>[2x]MAKKVTV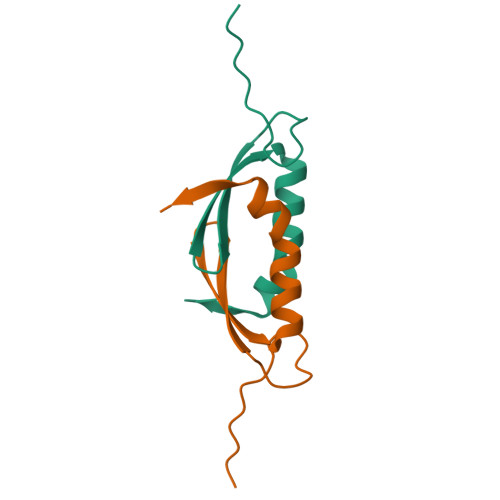TLVDDFDGSGAADETVEFGLDGVTYEIDLSTKNATKLRGDLKQWVAAGRRVGGR> MFEFTLMVVGESGLGKSTLINSLFLTDLYPERVIPGAAEKIERTVQIEASTVEIEERGVKLRLTVVDTPGYGD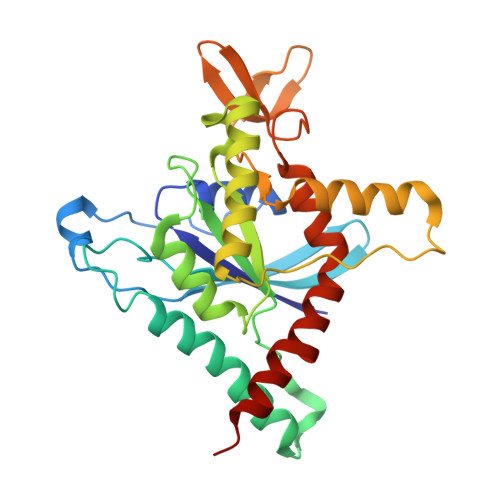AINCRDCFKTIISYIDEQFERYLHDESGLNRRHIIDNRVHCCFYFISPFGHGLKPLDVAFMKAIHNKVNIVPVIAKADTLTLKERERLKKRILDEIEEHNIKIYHLPDAESDEDEDFKEQTRLLKASIPFSVVGSNQLIEAKGKKVRGRLYPWGVVEVENPEHNDFLKLRTMLITHMQDLQEVTQDLHYENFRSERLKRGG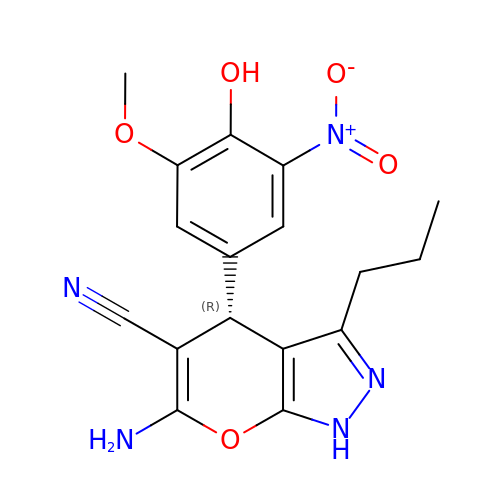(4R)-6-amino-4-(4-hydroxy-3-methoxy-5-nitrophenyl)-3-propyl-1,4-dihydropyrano[2,3-c]pyrazole-5-carbonitrile | C17 H17 N5 O5 | RWKXJNWNTFOJQN-ZDUSSCGKSA-N>MVVIANAHNELIHDAVLDYYGKRLATCSSDKTIKIFEVEGETHKLIDTLTGHEGPVWRVDWAHPKFGTILASCSYDGKVLIWKEENGRWSQIAVHAVHSASVNSVQWAPHEYGPLLLVASSDGKVSVVEFKENGTTSPIIIDAHAIGVNSASWAPATIEEDGEHNGTKESRKFVTGGADNLVKIWKYNSDAQTYVLESTLEGHSDWVRDVAWSPTVLLRSYLASVSQDRTCIIWTQDNEQGPWKKTLLKEEKFPDVLWRASWSLSGNVLALSGGDNKVTLWKENLEGKWEPAGEVHQ[4x];>GPHLQAPTWYGEPSPAAHWAFGGKLVQITPDGKGVSITNPKISGLESNTTLSEALKTKDFKPLINQRLVKVIDDVNEEDWNLLEKLSMDGTEEFLKEALAFDNDESGNIEQTISKNLVSGNIKSAVKNSLENDLLMEAMVIALDSNNERLKESVKNAYFAKYGSKSSLSRILYSISKREVDDLVENLDVSQWKFISKAIQNLYPNDIAQRNEMLIKLGDRLKENGHRQDSLTLYLAAGSLDKVASIWLSEFPDLEDK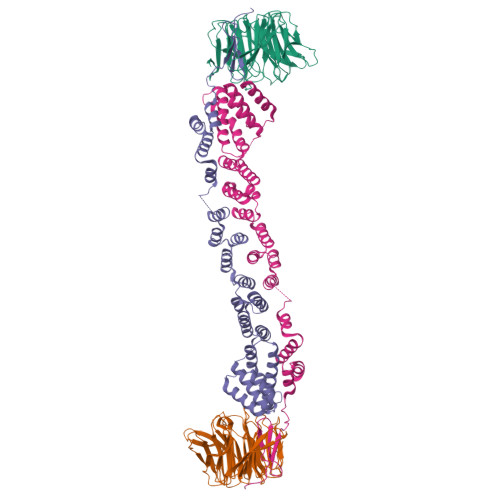LKKDNKTIYEAHSECLTEFIERFTVFSNFINGSSTINNEQLIAKFLEFINLTTSTGNFELATEFLNSLPSDNEEVKTEKARVLIASGK[4x]> GSHMSGKARLHYPVTRQGEQVDHYFGQAVADPYRWLEDDRSPETEAWVKAQNAVTQDYLAQIPYRAAIKEKLAASWNYAKEGAPFREGRYHYFFKNDGLQNQNVLWRQQEGKPAEVFLDPNTLSPDGTTALDQLSFSRDGRILAYSLSLAGSDWREIHLMDVESKQPLETPLKDVKFSGISWLGNEGFFYSSYDKPDGSELSARTDQHKVYFHRLGTAQEDDRLVFGAIPAQHHRYVGATVTEDDRFLLISAANSTSGNRLYVKDLSQENAPLLTVQGDLDADVSLVDNKGSTLYLLTNRDAPNRRLVTVDAANPGPAHWRDLIPERQQVLTVHSGSGYLFAEYMVDATARVEQFDYEGKRVREVALPGLGSVSGFNGKHDDPALYFGFENYAQPPTLYRFEPKSGAISLYRASAAPFKPEDYVSEQRFYQSKDGTRVPLIISYRKGLKLDGSNPTILYGYGGFDVSLTPSFSVSVANWLDLGGVYAVANLRGG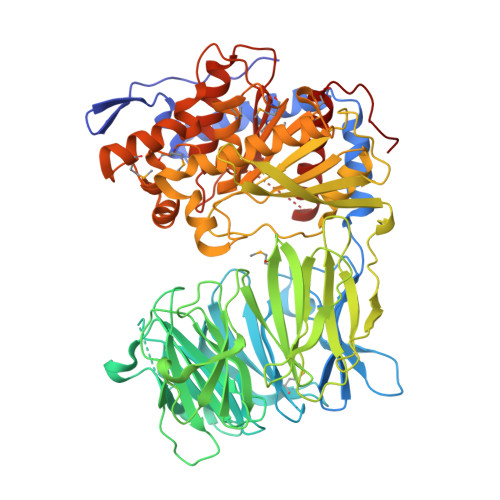GEYGQAWHLAGTQQNKQNVFDDFIAAAEYLKAEGYTRTDRLAIRGGSNGGLLVGAVMTQRPDLMRVALPAVGVLDMLRYHTFTAGTGWAYDYGTSADSEAMFDYLKGYSPLHNVRPGVSYPSTMVTTADHDDRVVPAHSFKFAATLQADNAGPHPQLIRIETNAGHGAGTPVAKLIEQSADIYAFTLYEMGYRELPRQP>[2x]ANPLYQKHIISINDLSRDDLNLVLATAAKLKANPQPELLK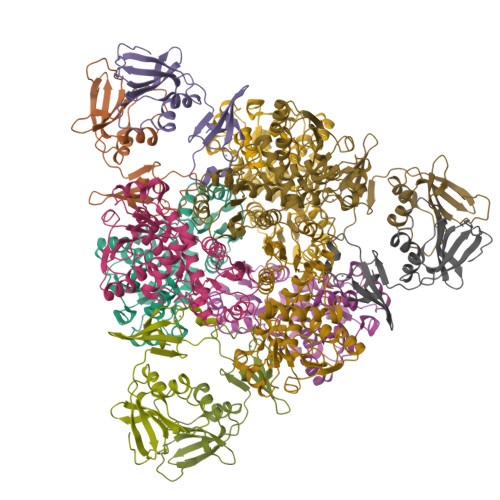HKVIASCFFEASTRTRLSFETSMHRLGASVVGFSDSANTSLGKKGETLADTISVISTYVDAIVMRHPQEGAARLATEFSGNVPVLNAGDGSNQHPTQTLLDLFTIQETQGRLDNLHVAMVGDLKYGRTVHSLTQALAKFDGNRFYFIAPDALAMPQYILDMLDEKGIAWSLHSSIEEVMAEVDILYMTRVQKERLDPSEYANVKAQFVLRASDLHNAKANMKVLHPLPRVDEIATDVDKTPHAWYFQQAGNGIFARQALLALVLNRDLVL;>[2x]MTHDNKLQVEAIKRGTVIAHIPAQIGFKLLSLFKLTETDQRITIGLNLPSGEMGRKDLIKIENTFLSEDQVDQLALYAPQATVNRIDNYEVVGKSRPSLPERIDNVLVCPNSNCISHAEPVSSSFAVRKRANDIALKCKYCEKEFSHNVVLAN> ALVKEEIQAKEYLENLNKELAKRTNVETEAAWAYGSNI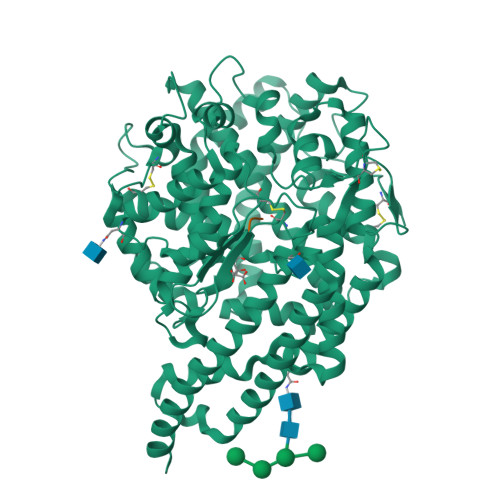TDENEKKKNEISAELAKFMKEVASDTTKFQWRSYQSEDLKRQFKALTKLGYAALPEDDYAELLDTLSAMESNFAKVKVCDYKDSTKCDLALDPEIEEVISKSRDHEELAYYWREFYDKAGTAVRSQFERYVELNTKAAKLNNFTSGAEAWLDEYEDDTFEQQLEDIFADIRPLYQQIHGYVRFRLRKHYGDAVVSETGPIPMHLLGNMWAQQWSEIADIVSPFPEKPLVDVSAEMEKQGYTPLKMFQMGDDFFTSMNLTKLPQDFWDKSIIEKPTDGRDLVCHASAWDFYLTDDVRIKQCTRVTQDQLFTVHHELGHIQYFLQYQHQPFVYRTGANPGFHEAVGDVLSLSVSTPKHLEKIGLLKDYVRDDEARINQLFLTALDKIVFLPFAFTMDKYRWSLFRGEVDKANWNCAFWKLRDEYSGIEPPVVRSEKDFDAPAKYHISADVEYLRYLVSFIIQFQFYKSACIKAGQYDPDNVELPLDNCDIYGSAAAGAAFHNMLSMGASKPWPDALEAFNGERIMSGKAIAEYFEPLRVWLEAENIKNNVHIGWTTSNKCVS;> RPPGFSPFR>MHHHHHHASMVRRDGKFVESKSRALFVESTEGALPSESDVVIIGGGIQGIMTAINLAERGMSVTILEKGEVAGEQSGRAYSQIISYQTSPEIFPLHHYGKILWRGMNEKIGADTSYRTQGRVEALADEKALDRAQEWIKTAKETAGFDVPLNTRIIKGEELSNRLVGAQTPWTVAAFEEDSGSVDPETGTPTLARYAKQIGVKIYTHCAVRGIETAGGKISDVVTEKGAIRTSNVVLAGGIWSRLFMGNMGVDLPTLNVYLSQQRV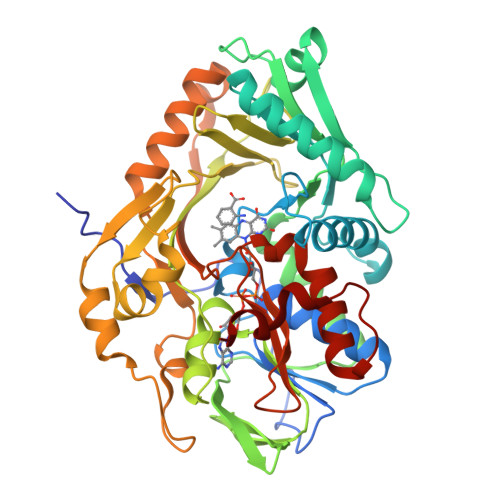SGVPGAPRGNVHLPNGIHFREQADGTYAVAPRIFTSSIVKDSFLLGPKFMHLLGGGELPLEFSIGEDLFNSFKMPTSWKLDEKSPFEQYRIATATQNTEHLDAVFQRMKTEFPVFEKSQIVERWGAVVSPTFDELPIISEVKEYPGLVINTATVWGMTEGPAAGEVTADIVTGKKPVIDPTPFSLDRFKK[2x]The ubiquitin-proteasome system (UPS) is a crucial regulatory pathway responsible for eliminating damaged or unnecessary proteins within cells. Central to this system is the proteasome, a molecular machine that selectively degrades proteins. A hydrophobic-tyrosine-any residue (HbYX) motif on the C-termini of proteasome-activating complexes independently triggers gate-opening of the 20S core particle for protein degradation; however, the causal allosteric mechanism remains unclear. The architecture of the archaeal 20S proteasome is conserved resembling the eukaryotic 20S, but its α and β rings are homoheptameric rather than heteroheptameric.

To determine the details of how the HbYX motif induces gate-opening in the archaeal 20S proteasome, we used 20S from Thermoplasma acidophilum (T20S) and incubated it with ZYA. Additionally, we noted a lack of density in the central channel showing the N-termini pointing up in the ZYA-T20S map, compared to the WT T20S map, clearly indicating a conformation that corresponds to the open-gate state. This ZYA-T20S structure resolves the N-termini of the α subunits up to Gly4, which include three N-terminal residues that have not been previously resolved. In the ZYA-T20S map, densities corresponding to ZYA bound to the α intersubunit pockets were clearly visible (in blue) and resembled the expected structure of this dipeptide. The carboxybenzyl group (i.e., Hb group) docks in a hydrophobic pocket, interacting with V24, L21, and A154, 3.7 Å, 4.3 Å and 3.6 Å away, respectively. Additionally, we noted the backbone of the dipeptide hydrogen bonding with the backbone of G80, V82, and ZYA’s C-terminal carboxylic group forming a salt bridge with the sidechain of K66, consistent with previous observations on the importance of K66 for HbYX-dependent gate-opening. The ZYA-T20S model also showed that the binding of ZYA to the intersubunit pocket shortens the distance between G19 on one subunit and K66 on the neighboring subunit by ~1 Å (essentially the walls of the intersubunit pocket are pulled together in the range of 1-2 Å), primarily due to a shift of K66 α carbon. Thus, the intersubunit “bridging” role ZYA plays leads to a K66 shift that promotes a rigid body rotation of the α subunits. In this T20S model, the T13 side chain occupies the space between Helices 0 and 2 and I12 is seen binding to a hydrophobic pocket created by the neighboring subunits N-termini comprising A11, I12, and V14. Interestingly, the ZYA-T20S model shows that T13 is pulled out of the pocket from under Helices 0 and now I12 binds into this same pocket, which is mostly hydrophobic, containing A11, I12, and V14 of the same subunit (Fig. 6a, e, I versus b, f, j). Simply put, I12 and T13 switch binding locations under Helix 0 to switch from the closed to the open state.

>[14x]GQMAYDRAITVFSPDGRLFQVEYAREAVKKGSTALGMKFANGVLLISDKKVRSRLIEQNSIEKIQLIDDYVAAVTSGLVADARVLVDFARISAQQEKVTYGSLVNIENLVKRVADQMQQYTQYGGVRPYGVSLIFAGIDQIGPRLFDCDPAGTINEYKATAIGSGKDAVVSFLEREYKENLPEKEAVTLGIKALKSSLEEGEELKAPEIASITVGNKYRIYDQEEVKKFL;>[14x]TTTVGITLKDAVIMATERRVTMENFIMHKNGKKLFQIDTYTGMTIAGLVGDAQVLVRYMKAELELYRLQRRVNMPIEAVATLLSNMLNQVKYMPYMVQLLVGGIDTAPHVFSIDAAGGSVEDIYASTGSGSPFVYGVLESQYSEKMTVDEGVDLVIRAISAAKQRDSASGGMIDVAVITRKDGYVQLPTDQIESRIRKLGLIL>[2x]SMAGCVVIVGSGVIGRSWAMLFASGGFQVKLYDIEQQQIRNALENIRKEMKLLEQAGSLKGSLSVEEQLSLISGCPNIQEAVEGAMHIQECVPEDLELKKKIFAQLDSIIDDRVILSSSTSCLMPSKLFAGLVHVKQCIVAHPVNPPYYIPLVELVPHPETAPTTVDRTHALMKKIGQCPMRVQKEVA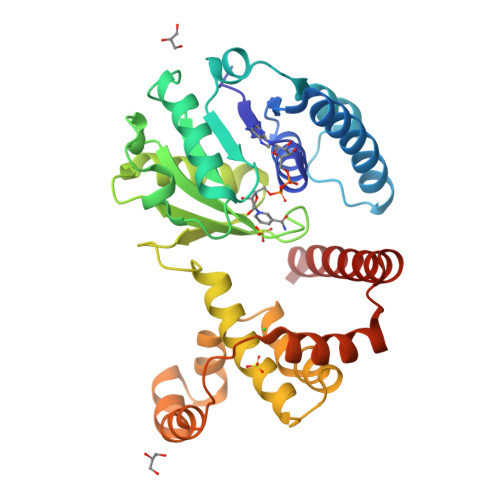GFVLNRLQYAIISEAWRLVEEGIVSPSDLDLVMSEGLGMRYAFIGPLETMHLNAEGMLSYCDRYSEGIKHVLQTFGPIPEFSRATAEKVNQDMCMKVPDDPEHLAARRQWRDECLMRLAKLKSQV> MLWLAATHRNRVAFQLFATPREPTASKAAAAARAAAEAVARSSTVSAPFTVQKQQRLLALLAASSSVADPSADLFRVHGLPGFSGFRPSSPPHLSKLFRGRVSRHLSCRRVNHLGRNNSGRITVRFRGAGHFRRLRFVDYKRGRKDIFGTVLRLEYDPNRSAHLALLQYDDGVLSYILA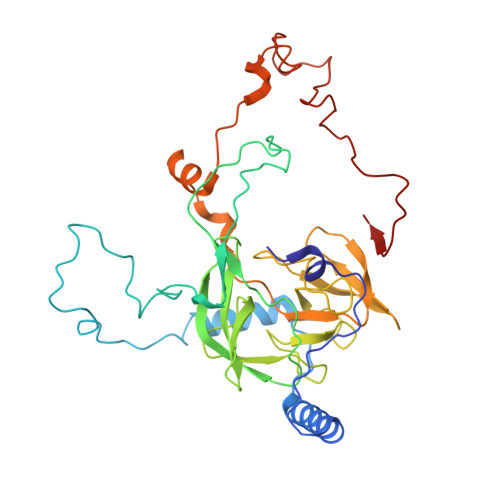TEVTRPGDRVVASKHASIAPGNCLPLGNIPVSTIVHNVELRPGAGGQIVRAGGCYATVVAKDRHFVTLKLSSTEVRRFPADCWATVGQVSNAAHAERIRGKAGVSYWMGERPRTRGKAMNPVDHPHGGGTGKKGLKRPPVSKWGILCKGYKTRAKKKPLGLIVRR> MYQNFVTKHDTAIQTSRFSVTGNV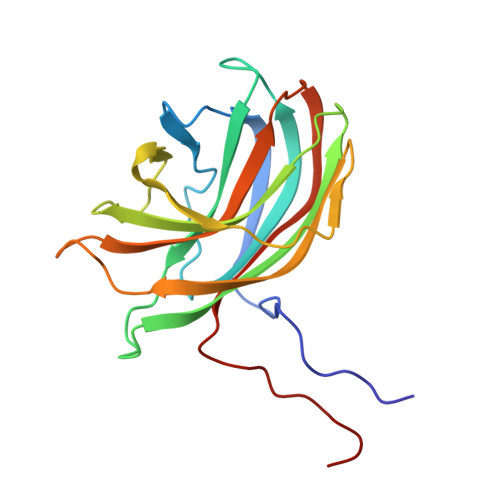IPAAPTGNIPVINGGSITAERAVVNLYANMNVSTSSDGSFIVAMKVDTSPTDPNCVISAGVNLSFAGTSYPIVGIVRFESASEQPTSIAGSEVEHYPIEMSVGSGGVCSARDCATVDIHPRTSGNNVFVGVICSSAKWTSGRVIGTIATTQVIHEYQVLQPLK> GSHMAGHSKWANTRHRKAAQDAKRGKIFTKIIRELVTAAKLGGGDPDANPRLRAAVDKALSNNMTRDTLNRAIARGVGGDDDANMETIIYEGYGPGGTAIMIECLSDNRNRTVAEVRHAFSKCGGNLGTDGSVAYLFSKKGV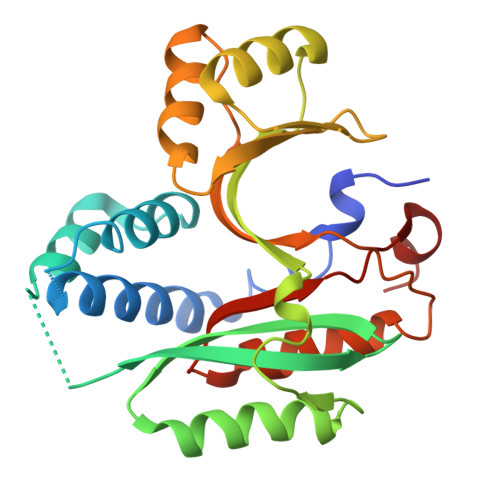ISFEKGDEDTIMEAALEAGAEDVVTYDDGAIDVYTAWEEMGKVRDALEAAGLKADSAEVSMIPSTKADMDAETAPKLMRLIDMLEDCDDVQEVYHNGEISDEVAATL>[2x]MVLIF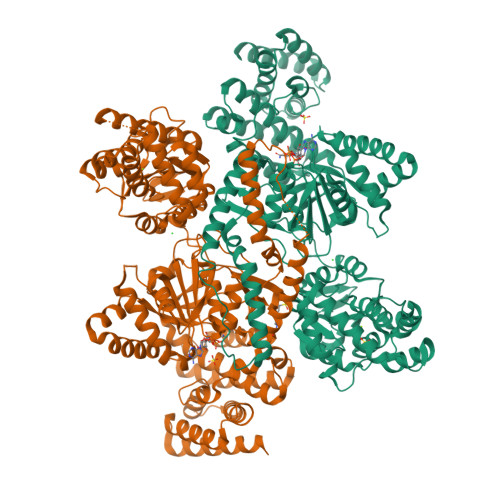HGKPVHGAIFDMDGTMFDTERLRFQTLQQASQELIGQEFSHEYLMQCLGLSATTAEKLAQRLYGVDVPYKEIRKRADEMELEHIRKHGVPIKKGLVQVLERLRKSGLRMAVATSSRRAIAEEYLINANVYKFFDVITCGDEVEQGKPHPEIFLKAASQLHLDANQCLMFEDSENGLTSAHTSKGLTILLKDIKEPNDEMLEKAHFYYDQMYDFLTDLDQFIPVMDMPEMQEPFPQSLNQLTVGIHGFGAIGGGYIAQILSHWDGYTKPKRIIASTRNSLFREAVNAFGTYSIRYGQFSYDERIENMSIVDSDNEQQMLEMYTHSSLIALCLPEQAIESESKIIAKGLYARFNSQLETCIEPLTFLIILNKVGAKYLVMKHLKEALLELTNDEDVTEHILKEHYFCDTVVNRMVSKLSNQNLYRQLRIKHNFLEQHLEDVEQEDQIEIEDCNKLTPDQLNQASIYVDNMRRNFQPGHILQSMDLILFHSETDMPIYVEKGSPLLEKLRQVVLVDQITDIQLIKNRLWNGVHAMLAWYASLMGYESIGVAMGDHLVKAFAENLIAEVKQGLAIVLPNYAKDLDRMSQSFLDSCEYAFKDPCQRVARDPLRKLNHNERVMASIAVNIRHDLPYKNLLKGAALGYAYAIQFLEIEETKAVEHLQQQIQNLDLSTAQRRQLEAELVQLIQYLFSEQGKQPLDIKSNNTKTTSTQYVAAALEHHHHHH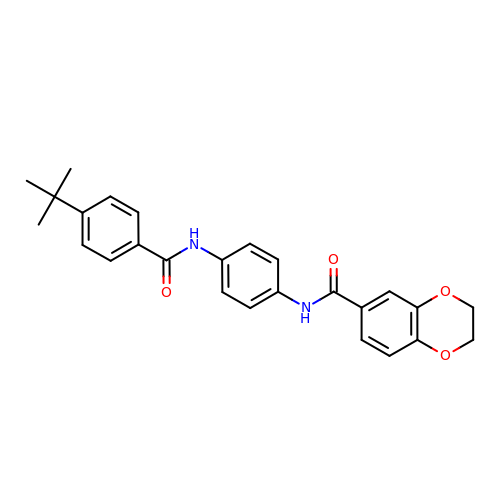~{N}-[4-[(4-~{tert}-butylphenyl)carbonylamino]phenyl]-2,3-dihydro-1,4-benzodioxine-6-carboxamide | C26 H26 N2 O4 | DRELUPFLXXDYEO-UHFFFAOYSA-N>MLIQHVQELIGHTPLMALPIEVPNHSHIYAKLEMFNPGGSIKDRLGAYLIEDGLQRGRVNAKTTIIEPTAGNTGIGLALATQAHHLRTILVVPEKFSMEKQVLMQALGAEIVHTPSEEGIKGAIRKAEALAATISNSYVPMQFKNPANPAAYYHTLAPEILADMPAPITAFVAGAGSGGTFAGVAAYLQAQDSATKAVVVEPEGSILNGGPAHAHRTEGIGVEFIPPFFDQVRIDQTLTIADNDAFAQVRHLARDHGLLI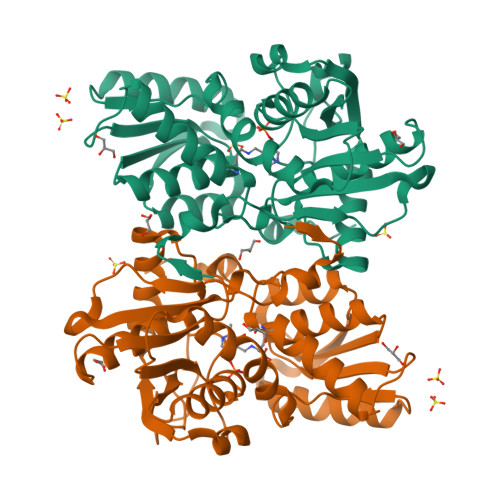GSSSGAALAASLQLATNLPANSHIVTIFPDSSERYLSQKIYTKLEHHHHHH[4x]>[2x]LTPDQQTLLHFIMDSYNKQRMPQEITNKILKEEFSAEENFLILTEMATNHVQVLVEFTKKLPGFQTLDHEDQIALLKGSAVEAMFLRSAEIFNKKLPSGHSDLLEERIRNSGISDEYITPMFSFYKSIGELKMTQEEYALLTAIVILSPDRQYIKDREAVEKLQEPLLDVLQKLCKIHQPENPQHFACLLGRLTELRTFNHHHAEM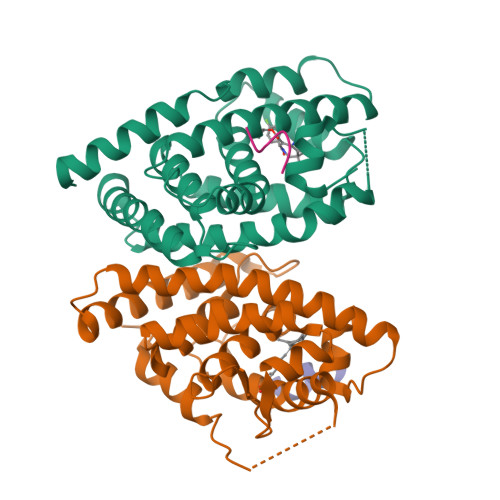LMSWRVNDHKFTPLLCEIWDVQ;>[2x]EDMPVERILEAELAVEPKTETYVEANMGLNPSSPNDPVTNICQAADKQLFTLVEWAKRIPHFSELPLDDQVILLRAGWNELLIASFSHRSIAVKDGILLATGLHVHRNSAHSAGVGAIFDRVLTELVSKMRDMQMDKTELGCLRAIVLFNPDSKGLSNPAEVEALREKVYASLEAYCKHKYPEQPGRFAKLLLRLPALRSIGLKCLEHLFFFKLIGDTPIDTFLMEMLEAP;>HKILHRLLQ[2x];>[2x]HKILHR> MTSNLIKFDDQNKVFHLHNKQISYLLSIEDGGTLSHLYFGGAVKNYNNQLKYPRLDRGFSGNLPESLDRTFSRDSLPKEYSSAGEMDFHTPATIVRNPDGSNALFLAYKSY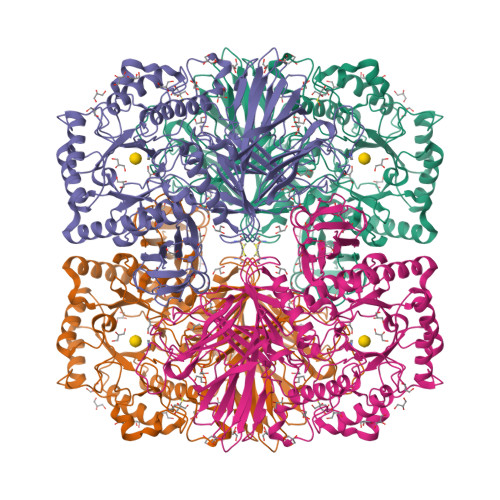KIEDGKPDLKGLPHSWTKEDDEAQTLIVTLEDKVSKLEYDLLYTIYRDRPVIVRSVQVHNHGEEAVYLEKVASMQMDYVDKDFEVITLPGAHANERRVQRENIGQGIKVFSSYRGTSSHQMNPFMALVDHDTNEFMGEAYGFALAYSGNHKFEVERDQFGQIHVNTGINDYNFKWKLNPNEEFQTPEVLMVYSDQGLNKMSQAFHSLIHERIMRSKFKDQIRPVLVNNWEATYFDFNEDKLKTIVDKAKKLGLEMFVLDDGWFGHRDDDNSSLGDWKVYKKKFPNGLGHFADYVHEQGLKFGLWFEPEMISYESNLYKEHPDYLMHVPGRKPCPSRNQYVLELGRKEVRDNIFEQMVKILDSKKIDYIKWDMNRSLSDIYESDLPADQQGEAYHRYVLGYYDLLNKLVTRYPDILFEGCSGGGGRFDVGQAYYTPQIWASDNTDAIERLKIQYGTSLVYPQSMMTSHVSVSPNEQNGRITPFNTRGAVAMWGDLGYELDLTKMSDEESDQVVKQVTEYKKIREVTQFGTLYRLKASASNQCAWMMVDSNKNEAVVTVVNVMAHAQPYCTKTKLAGLDPDKRYKNLETDEVFGGDELMHLGFYDPIERGDFKAKMYHFKAIN>MQQLNPSEISALIKQRIGDLDTSATAKNEGTIVMVSDGIVRIHGLADAMYGEMIEFDGGLFGMALNLEQDSVGAVVLGNYLSLQEGQKARCTGRVLEVPVGPELLGRVVDALGNPIDGKGPIDAKLTDAVEKVAPGVIWRQSVDQPVQTGYKSVDTMIPVGRGQRELIIGDRQTGKTAMAIDAIIAQKNSGIKCVYVAIGQKQSTIANVVRKLEETGAMAYTTVVAAAAADPAAMQYLAPYSGCTMGEYFRDRGEDALIIYDDLSKQAVAYRQISLLLRRPPGREAYPGDVFYLHSRLLERASRVSAEYVEKFTNGAVTGKTGSLTALPIIETQAGDVSAFVPTNVISITDGQIFLETSLFNAGIRPAVNAGISVSRVGGSAQTKIIKKLSGGIRTALAQYRELAAFAQFASDLDEATRKQLEHGQRVTELMKQKQYAPYSIADQAVSVYASNEGYMADVEVKKIVDFDAALIAYFRSEYAPLMKQIDETGDYNKDIEAAIKAGIESFKATQTY[3x];>[3x]MSSGRIIQIIGAVIDVEFERTSVPKIYDALQVDGTETTLEVQQQLGDGVVRTIAMGSTEGLKRGLTVTSTNAPISVPVGTATLGRIMDVLGRPIDEAGPVATEERLPIHRQAPSYAEQAASTDLLETGIKVIDLLCPFAKGGKVGLFGGAGVGKTVNMMELINNIAKAHSGLSVFAGVGERTREGNDFYHEMKDSNVLDKVAMVYGQMNEPPGNRLRVALTGLTMAEYFRDEKDENGKGRDVLLFVDNIYRYTLAGTEVSALLGRMPSAVGYQPTLAEEMGVLQERITSTKSGSITSIQAVYVPADDLTDPSPATTFAHLDATVVLSRDIASSGIYPAIDPLDSTSRQLDPLVVGQEHYEIARAVQNVLQRYKELKDIIAILGMDELAEEDKLVVYRARKIQRFFSQPFHVAEVFTGAPGKLVPLKETIRGFKGLLAGEYDHI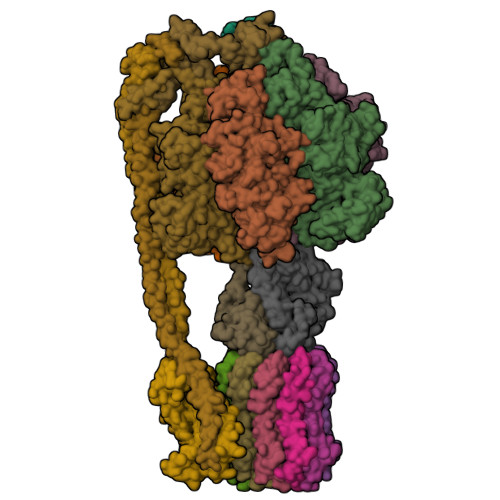PEQAFYMVGGIDEVIAKAEKL;>MELTLGLVAIASAILIAFGALGTAIGFGLLGGRFLEAVARQPELAPQLQTRMFLIAGLLDAVPMIGVGIGLFFIFANPFVG[10x];> MAAEEHALTSTEYIKHHLTNMTYGKMPDGTWKLAETAEEAHSMGFTAIHLDSMGWSIGLGVIFCLLFWIVARAANAGVPTKFQSAIEMIIEFVDSSVRDTFHGKSRLIAPLALTIFVWIFLMNLMDLIPVDWIPQVAAFVGANVFGMDPHHVYFKIVPSTDPNITLGMSLSVFVLILFYSIREKGVGGFVGELALNPFNPSNPVAKALLIPVNLILELVTFLARPISLALRLFGNMYAGELIFILIALLPFWIQWALSVPWAIFHILVITLQAFIFMMLTIVYLSMASEKH;>[2x]MNINLTLIGQAIAFAFFVAFCMKFVWPPLINAISERQRKIADGLNAAEKAKADLADAQAQVKQELDAAKAQAAQLIEQANRRAAQLIEEARTQAAAEGERIRQQAKEAVDQEINSAREELRQQVAALAVTGAEKILNQQVDAEAHNAMLSQLAAKL;> MAELLTLARPYAKAAFAYASEQGATDNWSNALQVLSAAVQDEAFSAYLNRPELTPAEQVKLFAKVLGEDQSQAVSNFLTLLADNDRLVLLPEIAAEYEQLKSQNNNNVDVVIESAFPLTAEQEQLLKSALEKRFNSTVTVSVEVKPELIAGVVIRAGDQVIDDSALNKLEKMRTRLLA;> MATMQCDVVSVKESIYSGAVTMLIAKGAGGELGILPGHAPLVTLLQPGPIRVLLENGTEEIVYVSGGVLEVQPHVVTVLADTAIRADNLDEAAILEARKNAEQLLANQKSDLDSAAALAALAETAAQLETIRKIKNRAQ;> MANLKEIRAKVASIKSTQKITRAMQMVAASKMRRAQERMAQGRPYADNMRRVIAHLVQANPEYKHRYMVDRPVKRVGYIIVSSDRGLAGGLNINLFKKVVQHVKAQQEQSIEVQFALIGQKAVSFFKNYGGKVLGATTQIGDAPSLEQLTGSVQVMLDAFDKGELDRIYLVSNGFVNAMTQKPKVEQLVPLAPAEEGDDLNRTYGWDYIYEPEAEELLNGLLVRYIESMVYQGVIENVACEQSARMVAMKAATDNAGQLIKDLQLIYNKLRQAAITQEISEIVGGAAAV>SNATDEKRPWMQNRRFEFIEWKLFWEGALNRSDLEETFEISTPQTSIDLRRYRELAGDNIEYDATDKTFKPTKGMKPSFLKVSADRLLLQLRALLTGALPRKEIWFREM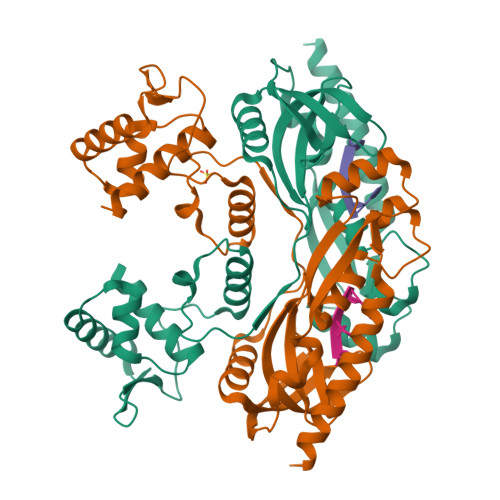PPMDMAPDIVRNVDPECLRLVLEAIRLKRSVEVRYQSLTNSRVREIAPHALAFDGYRWHVRAWACDRDDFRDFVLTRIDDIKPGSLANYDPEDDVEWTTVVTLDLRPHPGLTEEQALAIQRDYSMSDGMRKIDVRLSMAYYFIMRMNLDLEDLPPARAQLSLHNISDIRKSISEAKSESKRRIIARQNKD[2x]>MRGSHHHHHHGSDGDLVAFNKKEDKRTLWTTPDTSPNCKIDQDKDSKLTLVLTKCGSQILANVSLIVVAGKYKIINNNTQPALKGFTIKLLFDENGVLMESSNLGKSYWNFRNENSIMSTAYEKAIGFMPNLVAYPKPTAGSKKYARDIVYGNIYLGGKPDQPVTIKTTFNQETGCEYSITFDFSWAKTYV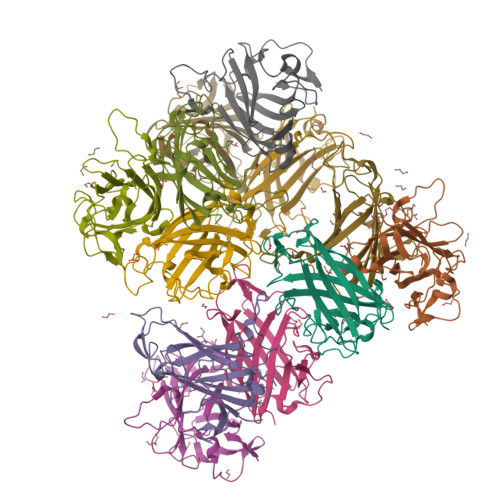NVEFETTSFTFSYIAQE[12x]> HHHHHHGSGTNVNDKVTASNFKLEKTTFDPNQSGNTFMAANFTVTDKVKSGDYFTAKLPDSLTGNGDVDYSNSNNTMPIADIKSTNGDVVAKATYDILTKTYTFVFTDYVNNKENINGQFSLPLFTDRAKAPKSGTYDANINIADEMFNNKITYNYSSPIAGIDKPNGANISSQIIGVDTASGQNTYKQTVFVNPKQR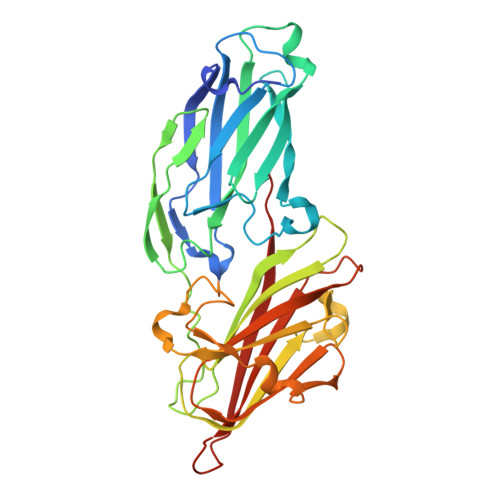VLGNTWVYIKGYQDKIEESSGKVSATDTKLRIFEVNDTSKLSESYYADPNDSNLKEVTDQFKNRIYYEHPNVASIKFGDITKTYVVLVEGHYDNTGKNLKTQVIQENVDPVTNRDYSIFGWNNENVVRYG>GSHMGHLYAINPDGTEKWRFKTGKAIEASPVIGEDGTIYVGSNDGHLYAINPDGTEKWRFKTGKAIEASPV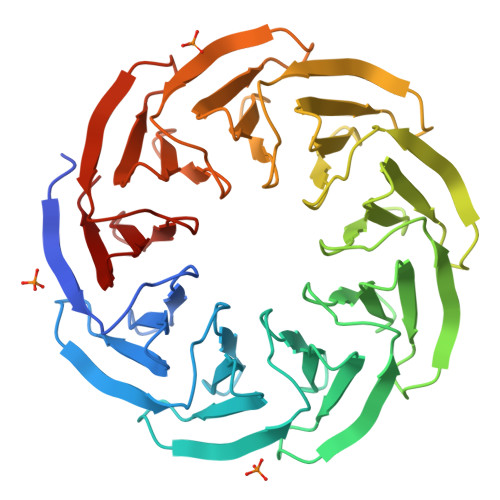IGEDGTIYVGSNDGHLYAINPDGTEKWRFKTGKAIEASPVIGEDGTIYVGSNDGHLYAINPDGTEKWRFKTGKAIEASPVIGEDGTIYVGSNDGHLYAINPDGTEKWRFKTGKAIEASPVIGEDGTIYVGSNDGHLYAINPDGTEKWRFKTGKAIEASPVIGEDGTIYVGSNDGHLYAINPDGTEKWRFKTGKAIEASPVIGEDGTIYVGSNDGHLYAINPDGTEKWRFKTGKAIEASPVIGEDGTIYVGSNDGHLYAINPDGTEKWRFKTGKAIEASPVIGEDGTIYVGSNDGHLYAINP[2x]> QAIKESYAFAVLGEPRYAFNFNHFDYVNPAAPKGGQITLSALGTFDNFNRYALRGNPGARTEQLYDTLFTTSDDEPGSYYPLIAESARYADDYSWVEVAINPRARFHDGSPITARDVEFTFQKFMTEGVPQFRLVYKGTTVKAIAPLTVRIELAKPGKEDMLSLFSLPVFPEKYWKDHKLSDPLATPPLASGPYRVTSWKMGQNIVYSRVKDYWAANLPVNRGRWNFDTIRYDYYLDDNVAFEAFKAGAFD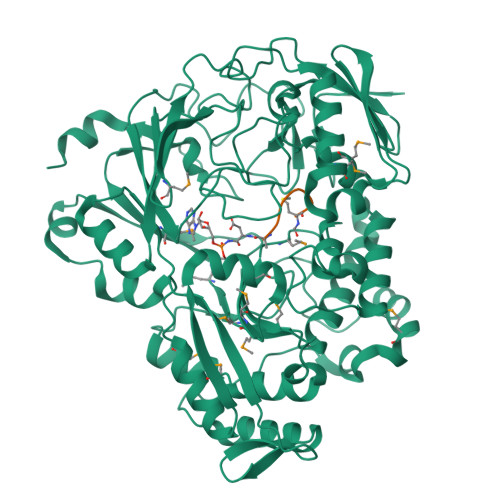LRMENDAKNWATRYTGKNFDKKYIIKDEQKNESAQDTRWLAFNIQRPVFSDRRVREAITLAFDFEWMNKALFYNAWSRTNSYFQNTEYAARNYPDAAELVLLAPMKKDLPSEVFTQIYQPPVSKGDGYDRDNLLKADKLLNEAGWVLKGQQRVNATEAQPLSFELLLPASSNSQWVLPFQHSLQRLGINMDIRKVDNSQITNRMRSRDYDMMPRVWRAMPWPSSDLQISWSSEYINSTYNAPGVQSPVIDSLINQIIAAQGNKEKLLPLGRALDRVLTWNYYMLPMWYMAEDRLAWWDKFSQPAVRPIYSLGIDTWWYDVNKAAKLPSASKQGE;> MRTGNAX> MAHHHHHHDYGIPTTENLYFQGSNPNYCFAGKTSSISDLKEVPRKNITLIRGLGHGAFGEVYEGQVSGMPNDPSPLQVAVKTLPEVCSEQDELDFLMEALIISKFNHQNIVRCIGVSLQSLPRFILMELMAGGDLKSFLRETRPRPSQPSSLAMLDLLHVARDIACGCQYLEENHFIHRDIAARNCLLTCPGPGRVAKIADFGMARDIYRASYYRKGGCAMLPVKWMPPEAFMEGIFTSKTDTWSFGVLLWEIFSLGYMPYPSKSNQEVLEFVTSGGRMD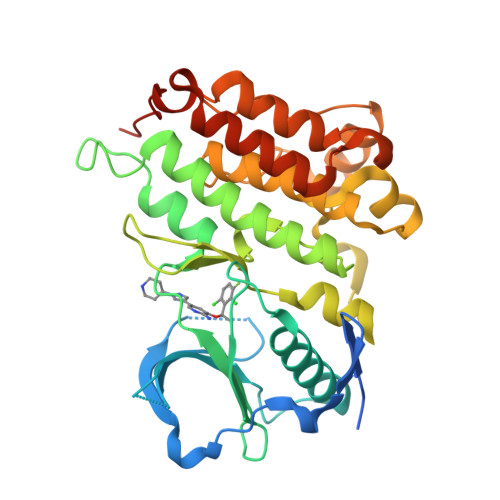PPKNCPGPVYRIMTQCWQHQPEDRPNFAIILERIEYCTQDPDVINTALPIEYGPLVEEEEKV> KLSPSPSS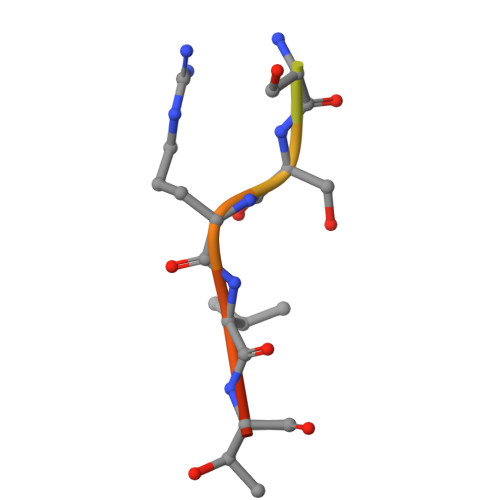RVTVS>[12x]MLPSAQVARLKPDPFPPSLSPIPHGAVTFAALAPCHNLPIFSSRQMLRDSLTYSHTSPTMSPQIANRFEASLDAQDIARISLFTLESGVILRDVPVAYKSWGRMNVSRDNCVIVCHTLTSSAHVTSWWPTLFGQGRAFDTSRYFIICLN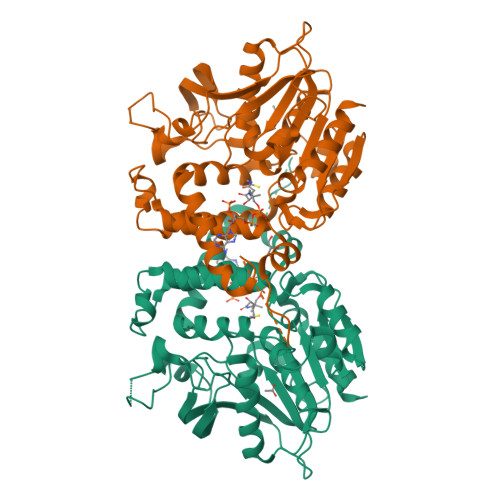YLGSPFGSAGPCSPDPDAEGQRPYGAKFPRTTIRDDVRIHRQVLDRLGVRQIAAVVGASMGGMHTLEWAFFGPEYVRKIVPIATSCRQSGWCAAWFETQRQCIYDDPKYLDGEYDVDDQPVRGLETARKIANLTYKSKPAMDERFHMAPGVQAGRNISSQDAKKEINGTDSGNSHRAGQPIEAVSSYLRYQAQKFAASFDANCYIAMTLKFDTHDISRGRAGSIPEALAMITQPALIICARSDGLYSFDEHVEMGRSIPNSRLCVVDTNEGHDFFVMEADKVNDAVRGFLDQSLM> MSQLEIRDLWASIDGETILKGVNLVVPKGEVHALMGPNGAGKSTLGKILAGDPEYTVERGEILLDGENILELSPDERARKGLFLAFQYPVEVPGVTIANFLRLALQAKLGREVGVAEFWTKVKKALELLDWDESYLSRYLNEGFSGGEKKRNEILQLLVLEPTYAVLDETDSGLDIDALKVVARGVNAMRGPNFGALVITHYQ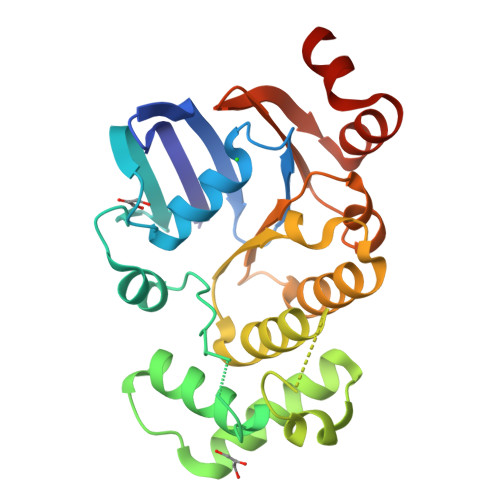RILNYIQPDKVHVMMDGRVVATGGPELALELEAKGYEWLKEKVKEGA>MRPPQFTRAQWFAIQHIDSDSSPSSSSRYCTIAMRAINNYRWRCKPVNTFVHEPLVDVQNVCFQEKVTCKNGQGNCYRSRFRMHITDCRLTNGSKYPNCRYRTRPGRRHIIVACEGSPYVPVHFDA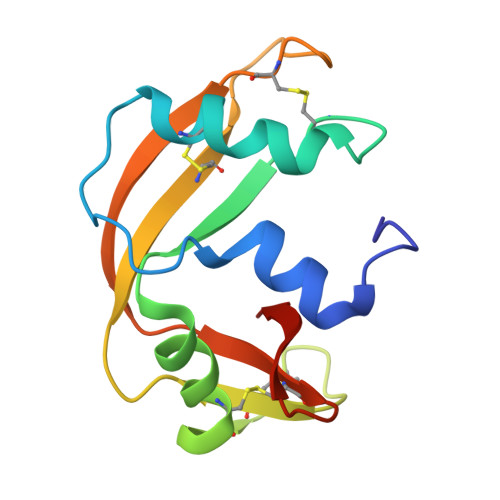SV[12x]>MLNEKAIQDVDLYFQNIHGPEGRLASNETFDIVPGLSKDGAVQYQTYQFNEAPKHLQKQVKAGRILMERFVAVASAAVNKKAPSNKEKYHYDIWKEVSNQLIPAFFTDPIKGEQNLNTTVKGVEVAKSVIQFAGNVIAGNVTGFATFLQNFGNGLSAEMNKTQANYNYLYAYSTHDLFQDTSGNVFYKPRFLIYGTHFKQEQKKIATSCASYQEVNLEFGVDTVGGTFRIEEYFSNETFKKKVDNFLDKYEGKAIDDADSYFDDIFNGVKPNKNYVYHHHHHH[2x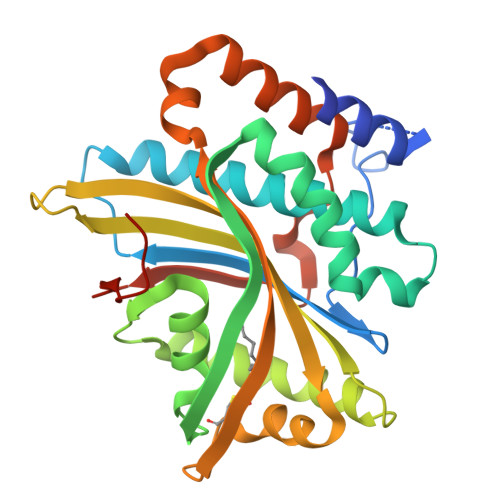]>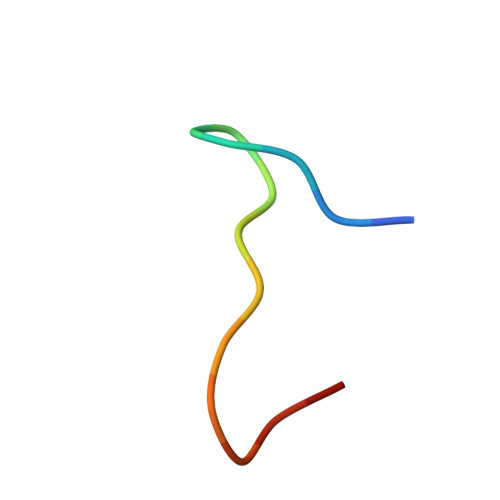 ACSFPKCPWVEGCAX> MAHHHHHHSAALEVLFQGPGYQDPNSVQALARPTSVDMGSKRRFSSEHPDPVETSIPEQAAEIAEELSKQHPLPSEEPLVHHDAGEFKGLQRHHTSAEEAQKLEDGKINPFTGREFTPKYVDILKIRRELPVHAQRDEFLKLYQNNQIMVFVGETGSGKTTQIPQFVLFDEMPHLENTQVACTQPRRVAAMSVAQRVAEEMDVKLGEEVGYSIRFENKTSNKTILKYMTDGMLLREAMEDHDLSRYSCIILDEAHERTLATDILMGLLKQVVKRRPDLKIIIMSATLDAEKFQRYFNDAPLLAVPGRTYPVELYYTPEFQRDYLDSAIRTVLQIHATEEAGDILLFLTGEDEIEDAVRKISLEGDQLVREEGCGPLSVYPLYGSLPPHQQQRIFEPAPESHNGRPGRKVVISTNIAETSLTIDGIVYVVDPGFSKQKVYNPRIRVESLLVSPISKASAQQRAGRAGRTRPGKCFRLYTEEAFQKELIEQSYPEILRSNLSSTVLELKKLGIDDLVHFDFMDPPAPETMMRALEELNYLACLDDEGNLTPLGRLASQFPLDPMLAVMLIGSFEFQCSQEILTIVAMLSVPNVFIRPTKDKKRADDAKNIFAHPDGDHITLLNVYHAFKSDEAYEYGIHKWCRDHYLNYRSLSAADNIRSQLERLMNRYNLELNTTDYESPKYFDNIRKALASGFFMQVAKKRSGAKGYITVKDNQDVLIHPSTVLGHDAEWVIYNEFVLTSKNYIRTVTSVRPEWLIEIAPAYYDLSNFQKGDVKLSLERIKEKVDRLNELKQGKNKKKSKHSKK;> MSPILGYWKIKGLVQPTRLLLEYLEEKYEEHLYERDEGDKWRNKKFELGLEFPNLPYYIDGDVKLTQSMAIIRYIADKHNMLGGCPKERAEISMLEGAVLDIRYGVSRIAYSKDFETLKVDFLSKLPEMLKMFEDRLCHKTYLNGDHVTHPDFMLYDALDVVLYMDPMCLDAFPKLVCFKKRIEAIPQIDKYLKSSKYIAWPLQGWQATFGGGDHPPKSDLEVLFQGPLGSMGLAATRTKQRFGLDPRNTAWSNDTSRFGHQFLEKFGWKPGMGLGLSPMNSNTSHIKVSIKDDNVGLGAKLKRKDKKDEFDNGECAGLDVFQRILGRLNGKESKISEELDTQRKQKIIDGKWGIHFVKGEVLASTWD

Prp43 (human DHX15) is an archetypical multitasking DEAH/RHA-box RNA helicase which functions during pre-mRNA splicing, spliceosome complex disassembly, ribosome biogenesis, cap-proximal mRNA methylation, and host defence during viral infections. In addition, G-patch cofactors boost Prp43-ATPase activity locally to drive processive RNA unwinding/annealing events. Functional studies indicate the requirement of the G-patch cofactor Pxr1 (PINX1 in humans) for early nucleolar pre-rRNA processing steps and a separate role in Rrp6-dependent 3′-end processing of small nucleolar RNAs (snoRNAs). In addition to the activating G-patch, we discover an inhibitory segment within Tma23 and Pxr1, I-patch, that restrains Prp43 ATPase activity.

A cryo-EM map of the Prp43:Pxr1GM complex at an overall resolution of 3.3 Å showed a defined density for Prp43 residues 52-718 and Pxr1 residues 122-136. No density for most of the N-terminus of Pxr1 (residues 1-121), which encompasses the G-patch (residues 29-72), was observed, supporting the idea that this region is highly flexible and only transiently interacts with Prp43 to stimulate its ATPase activity. Despite incubating the Prp43:Pxr1GM complex with the non-hydrolysable ATPγS before vitrification, the resulting density map showed only ADP bound to Prp43. We found that the I-patch is anchored onto the RecA2 domain through a set of hydrophobic contacts and extends towards the RecA1 domain. F126, within the -FKVGE- sequence (green lines), clusters with hydrophobic residues F437 and L439 within Prp43 on the RecA2 domain. The I-patch (residues 128-132) adopts a β-strand that is anti-parallel to the β-strand of Prp43 (residues 274-278) and extends the β-sheet from the centre of RecA2 domain. This involves contacts between L132 of Pxr1 and V274/L276 of Prp43. Another cluster at the C-terminal end of the I-patch involves the indole ring of W136 and the side chains of R270 and Y272 of Prp43, present within the loop that connects RecA1 with the RecA2 domain. We found that the RNA-binding tunnel of the Prp43:Pxr1GM complex adopts an open conformation in contrast to the activated closed Prp43:G-patch complexes (DHX15:NKRFG; PDB:6SH625). In this conformation, the C-terminal Ratchet and the OB fold domains are rotated with respect to the RecA-like domains resulting in the repositioning of the OB fold domain by ∼24 Å as compared to the G-patch-bound closed conformation.>MTYEAFVELVERLWEEVPEDFKRGLQGVHVFPEAKPEPGLEGVWRLGEYLDPGPPSAFGGFEDLGRHIALYYGSFLEVAGEGFDWEAEVWETMLHELRHHLESLAGRDDLVQEDLRRLDAFRRGGPSGEG[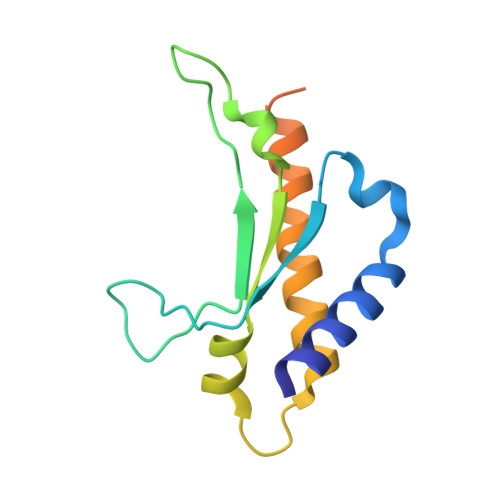2x]> MIIPALDLIGGTVVRVVRLHQGDYARLRDYGNDPLP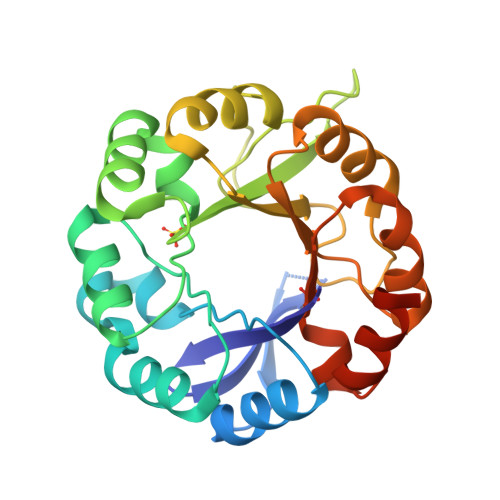RLQDYAAQGAGVLHLVDLTGAKDPAKRQIPLIKTLVAGVNVPVQVGGGVRTEEDVAALLKAGVARVVLASTAVKSPDVVKGWFERFGAQALVLALDVRIDEHGTKQVAVSGWQENSGVSLEQLVETYLPVGLKHVLCTDISRDGTLAGSDVSLYEEVCARYPQIAFQSSGGIGDIDDIAALRGTGVRGVIVGRALLEGKFTVKEAIQCWQNVKGHHHHHH> QLTPTFYRSTCPNVTSIVRGVIQDALQTDLRIPASLIRLHFHDCFVNGCDGSLLLDNSDTIESEKQAAPNNNSARGFDVVDNIKTAVENACPGVVSCADILTIAAEQSVWLSGGPSWPVPLGRRDSLTANRTLANQTLPSPFLT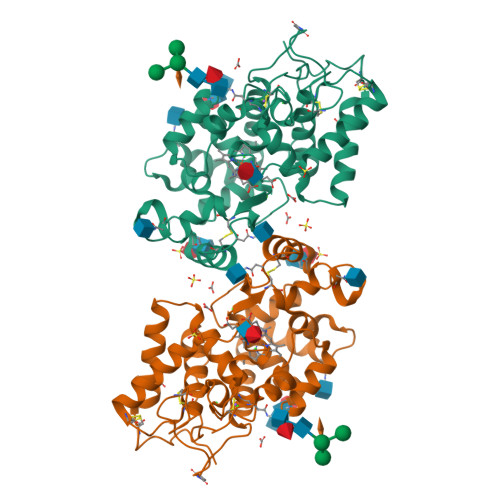LDQLKTDFSDQGLNTTDLVALSGAHTFGRAQCQFFSQRLYNFSATGSPDPTLNTTLLETLRNICPQGGNGSTITNLDQTTPDAFDNKYFSNLQTQYGILQTDQELFSTKGANTTAIVTKFSANQSAFFNSFVASMIKMGNIGVLTNDEGEIRSNCRSVNGGA> GEIAIYWGQDGGEGSLRETCDTDDYDIINIGFLTTFGHSTTPILNLTKHCNPATSACKFLSSEISYCKSKGIKVFLSLGGGTGNYYLSSRDDAASVAQYLWNNFLGGQS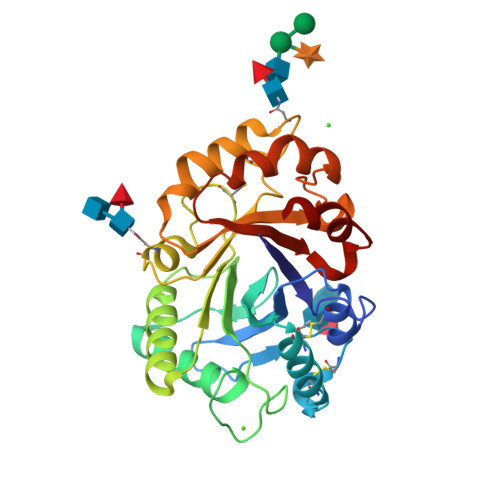ESRPLGDESLDGIDFDIEDGSNDYYDTLAEQLWILGGRSGSNVYLAAAPACEFPDYYLREAINTSLFDYVWVQFYNNPRCHYLGNATNLLNSWNNDWSTILTDDLFLGLPAAPQAAPGGGFIEADDLISEVLPTIKATYDYGGVMLWSKYYDDDYSSKIKPDV> MDELVKALERAGYLLTPSAYYLLVDHFKEGKFSLVELVKFAKSKGVFIIDGDLAYEFLQFLGLGVPQEIKESYISTGEEAEKTVESQETRASELEEGGVSQVSSGELQELKEESPEISTTEEEIGGLELVQSSISTGSEVEYNNGENGESVVVLDKYGYPILYAPEEIGEEKEYSKYEDVVIEWNPSVTPVQIEKNYEVKFDVRQVKLRPPKVKNGSGKEGEIIVEAYASLFKSRLSKLKRILRENPEISNVVDIGKLNYVSGDEEVTIIGLVNSKRETNRGLIFEVEDKTGIVKVFLPKDSEDYREAFKVLPDAVVAFKGFYSKKGIFFANKFYLPDVPLYRKQKPPLEEKVYAILISDIHVGSREFCEKAFLKFLEWLNGHVESKEEEEIVSRVKYLIIAGDVVDGIGIYPGQYSDLVIPDIFDQYEALANLLANVPEHITMFIGPGNADAARPAIPQPEFYKEYAKPIYKLKNAIIISNPAVIRLHGRDFLIAHGRGIEDVVSFVPGLTHHKPGLPMVELLKMRHLAPTFGGKVPIAPDPEDLLVIEEVPDLVQMGHVHVYDAVVYRGVQLVNSATWQAQTEFQKMVNIVPTPAKVPVVDVESARVVKVLDFSGWC;> GTGDGSELPKEMEEYFEMLQREIDKAYEIAKKARAQGKDPSLDVEIPQATDMAGRVESLVGPPGVAKRIRELVKEYGKEIAALKIVDEIIEGKFGDLGSREKYAEQAVRTALAILTEGIVSAPIEGIANVKIKRNTWADNSEYLALYYAGPIRSSGGTAQALSVLVGDYVRRKLGLDRFKPSEKHIERMVEEVDLYHRAVTRLQYHPSPEEVRLAMRNIPIEITGEATDDVEVSHRDVPGVETNQLRGGAILVLAEGVLQKAKKLVKYIDKMGIEGWEWLKEFVEAKEKGEPKEEGKEESLAESTLEETKVEVDMGFYYSLYQKFKEEIAPSDKYAKEVIGGRPLFSDPSKPGGFRLRYGRSRASGFATWGINPATMILVDEFLAIGTQLKTERPGKGAVVTPVTTIEGPIVKLKDGSVLRVDDYNLALKVREDVEEILYLGDAVIAFGDFVENNQTLLPA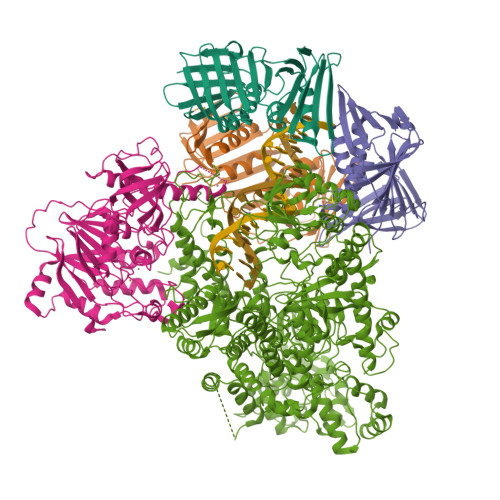NYCEEWWILEFVKALKEIYEVHLEPFTENEEESIEEASDYLEIDPEFLKEMLRDPLRVKPPVELAIHFSEVLGIPLHPYYTLYWNSVEPKDVEKLWRLLKNYAEIEWSNFRGIKFAKKIVISQEKLGDSKRTLELLGLPHTVRDGNVIVDYPWAAALLTPLGNLNWEFMAKPLYATIDIINENNEIKLRDRGISWIGARMGRPEKAKERKMKPPVQVLFPIGLAGGSSRDIKKAAEEGKVAEVEIAFFKCPKCGHVGPEHLCPNCGTRKELLWVCPRCNAEYPESQAEGYNYTCPKCNVKLRPYAKRKIRPSELLNRAMENVKVYGVDKLKGVMGMTSGWKMPEPLEKGLLRAKNDVYVFKDGTIRFDATDAPITHFRPREIGVSVEKLRELGYTHDFEGKPLVSEDQIVELKPQDIILSKEAGRYLLKVAKFVDDLLEKFYGLPRFYNAEKMEDLIGHLVIGLAPHTSAGIVGRIIGFVDALVGYAHPYFHAAKRRNCDGDEDAVMLLLDALLNFSRYYLPEKRGGKMDAPLVITTRLDPREVDSEVHNMDIVRYYPLEFYEATYELKSPKELVGVIERVEDRLGKPEMYYGLKFTHDTDDIALGPKMSLYKQLGDMEEKVRRQLEVAKRIRAVDEHGVAEKILNSHLIPDLRGNLRSFTRQEFRCVKCNTKFRRPPLNGKCPVCGGKIVLTVSKGAIEKYLGTAKMLVTEYNVKNYTRQRICLTERDIDSLFENVFPETQLTLIVNPNDICQRLVMARTGEVNKSGLLENLSNGSKKTEKAEKAEKPRKKSDEKPKKKRVISLEEFFSRKSK;>MRGSHHHHHHGSMPFEIVFEGAKEFAQLIETASRLIDEAAFKVTEEGISMRAMDPSRVVLIDLNLPASIFSKYEVDGEETIGVNMDHLKKVLKRGKAKETLILRKGEENFLEISLQGTATRTFKLPLIDVEEIEVDLPELPFTAKVVILGDVIKEAVKDASLVSDSMKFIAKENEFTMRAEGETQEVEVKLTLEDEGLLDIEVQEETKSAYGISYLSDMVKGLGKADEVTIKFGNEMPMQMEYYIRDEGRLIFLLAPRVEE[3x]>[4x]MAHHHHHHMTASAEFNGAIAVVTGAGSGIGRACAELLSRSGANVIVADRDIEAATRVARATGGKTLVLDVGEDASVTAAANEVRARYGVADVLVNCAGVLQRTLPPGELAQREWDVVSRIDLRGTYLCCAAFGAPMADRRRGSIVNIASVAGMRSGPLHAYGPAKAGVISLTETLAGEWGPKGVRVNC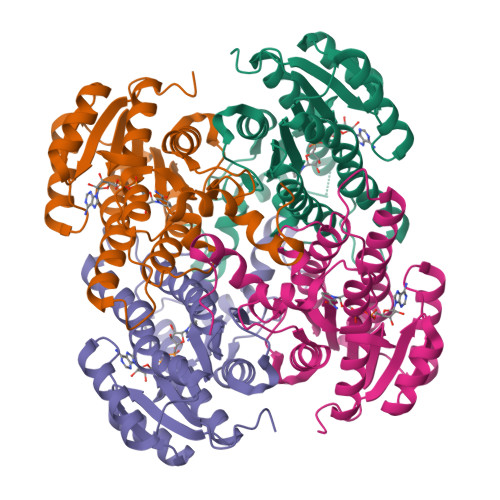VSPGFTQTPALERGFTTHTLKADVLRDAAALGHIVSANEIAEAVVFLASERASAITGVNLPVDAGYLIAGSWAAYGGLRRESAGQD(2~{R},3~{S},4~{S},5~{R},6~{S})-2-(hydroxymethyl)-6-[(2~{R},3~{R},4~{S},5~{R},6~{S})-2-(hydroxymethyl)-6-[(2~{R},3~{R},4~{S},5~{R},6~{R})-2-(hydroxymethyl)-3,5-bis(oxidanyl)-6-[4-(pyridin-2-ylmethoxymethyl)-1,2,3-triazol-1-yl]oxan-4-yl]oxy-3,5-bis(oxidanyl)oxan-4-yl]oxy-oxane-3,4,5-triol | C27 H40 N4 O16 | 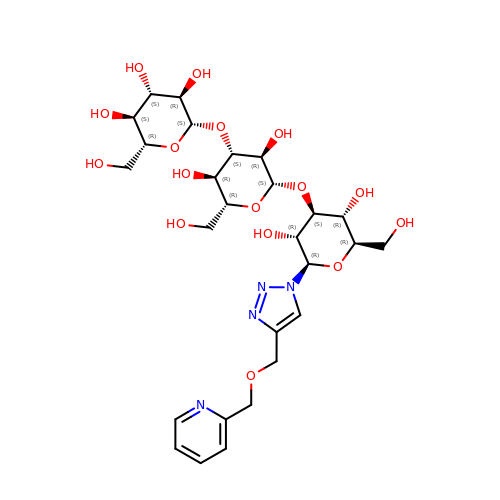GZCRLDXRIWVPBY-FLQYNTDFSA-N> NSEPSAPATISDNIYTTLYSSYPCTKIMTSDGQFGCSSKHGGNSGILYLIDDDESYNNYFSYSQQKDIIVVLDTNYFNSTSVLNLHNKSKIEGIIVLTDTKKTYPYSPDSRYPNKIYGLYPNSNLEWNPNADGFTYFSFPFPIFAIDNQT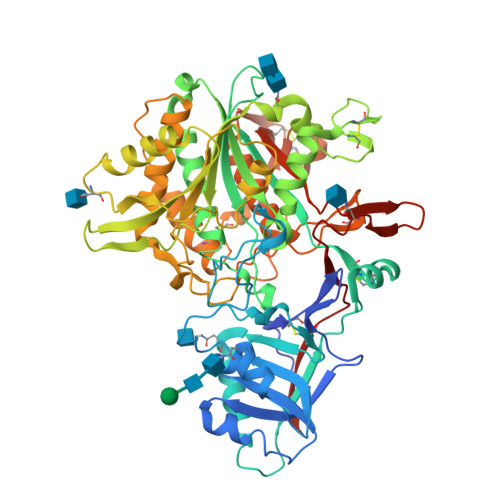SVAIRNVSKHNRDGQYPAWGAELDSFMQGAINSETCLRRGFCEPVGGQSIWSSFSSKIDKEKEIILVMLPFDTTAFFRDLSIGADQSSFATVTLLSVIKSLAAVDRSSWNKEVVFAFWNAERWGYVGSEYFINDLLNFQCKTYNSDKSKCIDPPRADLAFQTQINFTKISTIIELNQIGRAQLDKNLGKYSLYLHTAGTKTSSVTDILDQVASSYENSTITFKPTTQTELPPSSSMSFLKKTNKIPVVVITDHDYKYSNPYYGYEQDDNENVLGSTLNDIVYILSTFIDRIAGGNNNITIDKNFINILYPCFTSSITCFNILMKTYPLNEVPNFYSSVFGTSLTTTLSPYETKLIHRLLYSITQYNSTLTNCTSDNDCPSSLCYSGQCVSSNTHLHNALSLGFDFDTSKNVWKIVNSSYPIFTESNWDYTALKVFKIGNSTTE>[4x]MEKLRFPKDFIFGTATAAYQIEGAYKEDEKGESIWDRFSHIPGNVAKMHNGDIACDHYHRYKEDVQLLKSLGIKSYRFSIAWPRIFPKGFGEINQKGIQFYRDLIDELIKNDIEPAITIYHWDLPQKLQDIGGWANPQVADYYVDYANLLFREFGDRVKTWITHNEPWVASYLGYALGVHAPGIKDMKMALLAAHNILLSHFKAVK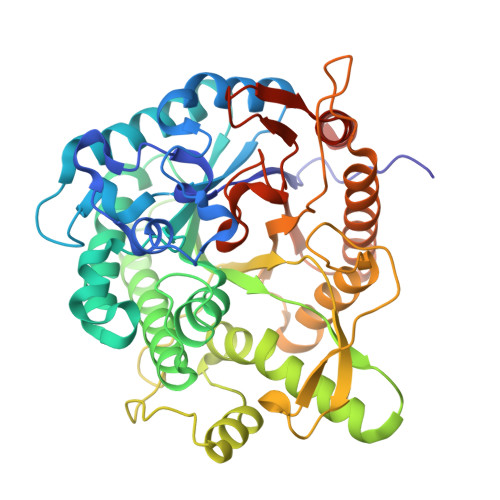AYRELEQDGQIGITLNLSTCYSNSADEEDIAAAHRSDGWNNRWFLDAALKGTYPEDMIKIFSDTNIMPELPKELFTEVFETSDFLGINYYTRQVVKNNSEAFIGAESVAMDNPKTEMGWEIYPQGLYDLLTRIHRDYGNIDLYITENGAAFNDMVNRDGKVEDENRLDYLYTHFAAALSAIEAGVPLKGYYIWSFMDNFEWAEGYEKRFGIVHVNYKTQERTIKKSAYWYKELIERSNKLEHHHHHH> GSHMTKYKYTVEESERFNKHGIDLTVYGQVDPSATVVRVSVERGQFQEFFNVRSSYTYYVVSGQGVFYLNSEAVPAGATDLITVPPNTRIHYFGSMEMVLTVAPAFNEQDERHVRFISESESPY

In pacidamycin 3, biosynthesis the 3′‐deoxy moiety is mediated by Pac13, an enzyme found to catalyze the key dehydration of uridine‐5′‐aldehyde 1 to form 3′‐deoxy‐3′,4′‐didehydrouridine‐5′‐aldehyde 2. In stark contrast to most characterised dehydratases, Pac13 is small (121 aa), monomeric, co‐factor independent and utilises a non‐activated nucleoside, rather than a free monosaccharide, as a substrate. Pac13 is the only monomeric, metal‐free cupin dehydratase characterised to date. We demonstrate here that the reaction most likely proceeds via an E1Cb mechanism, with H42 acting as an active site base, however, unlike many other dehydratases, no metal or cofactor is required for activity.

Mutants E108Q, K16R, H42Q, Y55F and Y89F were produced and purified, affording diffracting crystals of the same morphology and space group as wt Pac13, which raised our confidence that the mutants folded correctly and that the effects seen are specific to interactions with each mutated residue rather than global effects on protein folding and structure. The mutation of H42 to a Q completely abolished activity, further supporting our hypothesis that H42 acts as a base for the abstraction of the 4′ proton and possibly for the protonation of the 3′ hydroxy group. KGaAThe biochemical data were in accordance with the data obtained from structural analysis of the mutants. In the H42Q–uridine complex, the critical interactions between 5′ OH and Y55 and Y89 remained the same as in the WT‐uridine structure, additionally the hydrogen bond between K16 and E108 with 2′‐OH, as well as the π‐stacking of the uracil ring with F103 are all preserved. Q42 appears to have the same distance from the 4′ proton and the overall fold of the protein does not seem to be impacted, all of which suggests that the H42Q mutation affects the key catalytic step and not substrate binding.(3R)-1-(cyclopropylmethyl)-3-methyl-3-(4-methylsulfanylphenoxy)pyrrolidine 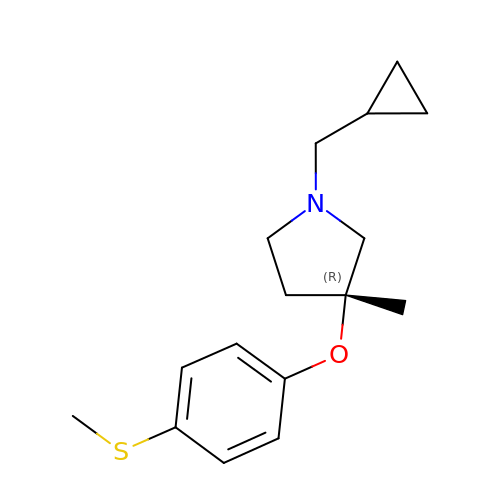| C16 H23 N O S | NBLYVOKOJMLIRY-MRXNPFEDSA-N> GASEIAALEKEIAALEKEIAALEKEISKQEKFYNDTYNTVCKELLRSRRLENSIIEQKGTMRVYAYVMEQNLPENLLFDYENGVITQGLSEHVYKFNRVIPHLKVSEDCFFTQEYSVYHDMALNQKKNFNLISLSTTPHGSLRESLIKFLAEKDTIYQKQYVITLQFVFLSDDEFSQDMLLDYSHNDKDS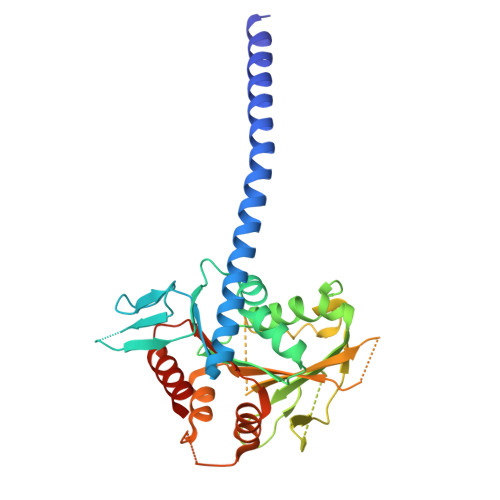IKLKFEKHSISLDSKLVIIENGLEDLPLNFSADEHPNLPHSGMGIIKVQFFPRDSKSDGNNDPVPVDFYFIELNNLKSIEQFDKSIFKKESAETPIALVLKKLISDTKSFFLLNLNDSKNVNKLLTISEEVQTQLAKRKKKLT>[4x]MIKLCREVWIEVNLDAVKKNLRAIRRHIPHKSKIMAVV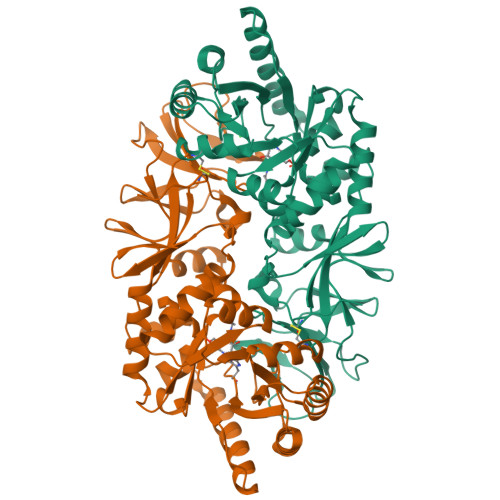KANGYGHGSIEVARHALEHGASELAVASVEEGIVLRKAGITAPILVLGFTSLSCVKKSAAWNITLSAFQVDWMKEANEILEKEASANRLAIHINVDTGMGRLGVRTKEELLEVVKALKASKFLRWTGIFTHFSTADEPDTTLTKLQHEKFISFLSFLKKQGIELPTVHMCNTAAAIAFPEFSADMIRLGIGLYGLYPSAYIKQLNLVKLEPALSLKARIAYVKTMRTEPRTVSYGATYIAEPNEVIATLPIGYADGYSRALSNRGFVLHRGKRVPVAGRVTMDMIMVSLGENGEGKQGDEVVIYGKQKGAEISVDEVAEMLNTINYEVVSTLSRRIPRFYIRDGEIFKVSTPVLYV N-[4-(2-amino-1,3-thiazol-4-yl)phenyl]acetamide | C11 H11 N3 O S | 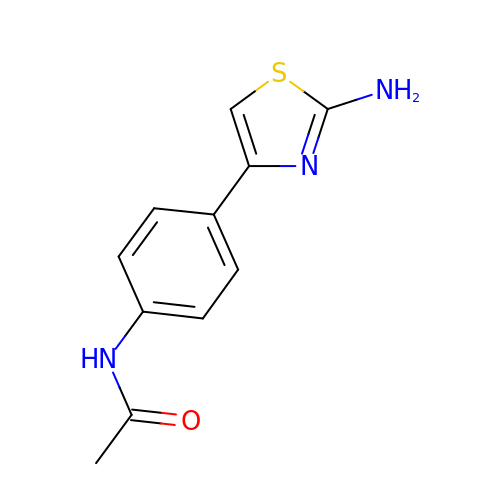VBBNSESFUHRMJU-UHFFFAOYSA-N>[3x]MRCVGVGNRDFVEGLSGATWVDVVLEHGGCVTTMAKNKPTLDIELQKTEATQLATLRKLCIEGKITNITTDSRCPTQGEAVLPEEQDQNYVCKHTYVDRGWGNGCGLFGKGSLVTCAKFQCLEPIEGKVVQYENLKYTVIITVHTGDQHQVGNETQGVTAEITPQASTTEAILPEYGTLGLECSPRTGLDFNEMILLTMKNKAWMVHRQWFFDLPLPWASGATTETPTWNRKELLVTFKNAHAKKQEVVVLGSQEGAMHTALTGATEIQNSGGTSIFAGHLKCRLKMDKLELKGMSYAMCTNTFVLKKEVSETQHGTILIKVEYKGEDAPCKIPFSTEDGQGKAHNGRLITANPVVTKKEEPVNIEAEPPFGESNIVIGIGDNALKINWYKKGSSIGKMFEATARGARRMAILGDTAWDFGSVGGVLNSLGKMVHQIFGSAYTALFSGVSWVMKIGIGVLLTWIGLNSKNTSMSFSCIAIGIITLYLGAVVQA;>SVALAPHVGMGLDTRTQTWMSAEGAWRQVEKVETWALRHPGFTILALFLAHYIGTSLTQKVVIFILLMLVTPSMT[3x]

The nucleocapsid is surrounded by a bilayer lipid membrane and on the outside of the membrane are the 180 pairs of envelope (E) and membrane (M) proteins. The E and M proteins are arranged with icosahedral symmetry with each asymmetric unit containing three pairs of E and M heterodimers. The E protein ectodomain consists of three domains: DI, DII and DIII121314. E protein plays an important role in virus entry into host cell as it binds to receptors and facilitates fusion of the virus to the endosomal membrane.

To increase the precision of the fit of E protein structures on DENV3 surface, we also determined the cryo-EM structure of uncomplexed mature DENV3 to 6 Å resolution. The densities of the helical ridges on the transmembrane helices are visible. DENV3 used in this structure determination was grown in C6/36 cells at 28 °C and kept at 4 °C before freezing on cryo-EM grids. The DENV3 E protein has two residues deleted in the EoFo loop compared with DENV1, 2 and 4. Superposition of cryo-EM structures of uncomplexed DENV3 at 28 °C and 37 °C showed similar structures. Therefore, unlike the DENV2 New Guinea C strain3233, the E protein layer of the uncomplexed DENV3 863DK strain does not undergo irreversible conformational changes when exposed to 37 °C. A homology model of the variable region of the Ab heavy and light chains, and the 6-Å resolution cryo-EM structure of the uncomplexed DENV3 863DK strain were then fitted into the 9-Å cryo-EM Fab-DENV structure. The DENV3–Fab 5J7 complex structure displayed a very similar E protein conformation as uncomplexed DENV3. Superposition of the Cα chains of E proteins of the Fab complex and uncomplexed cryo-EM structures showed a root mean square deviation value of 1.08 Å.> GPMGRKKIQITRIMDERNRQVTFTKRKFGLMKKAYELSVLCD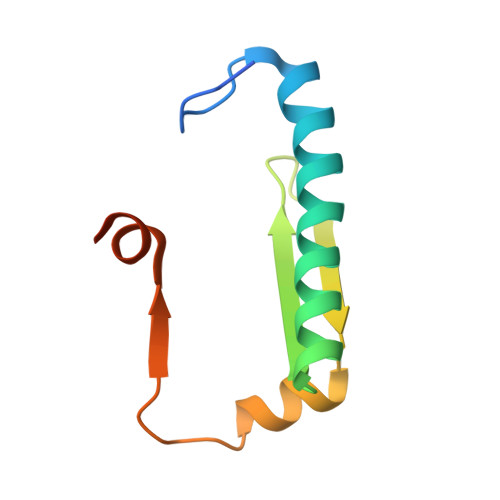CEIALIIFNSSNKLFQYASTDMDKVLLKYTEYNEPHESRTNSDIVEALNKKEHRG> MSRSKRDNNFYSVEIGDSTFTVLKRYQNLKPIGSGAQGIVCAAYDAILERNVAIKKLSRPFQNQTHAKRAYRELVLMKCVNHKNIIGLLNVFTPQKSLEEFQDVYIVMELMDANLCQVIQMELDHERMSYLLYQM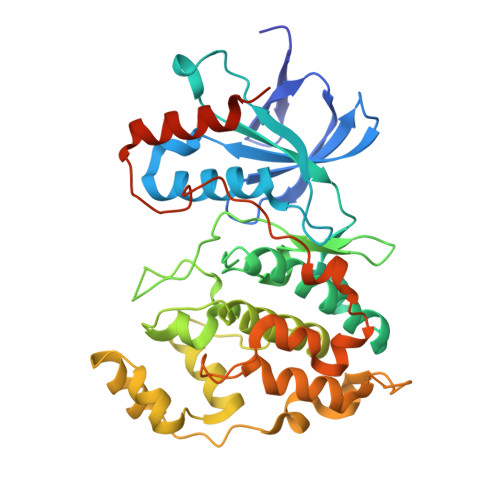LCGIKHLHSAGIIHRDLKPSNIVVKSDCTLKILDFGLARTAGTSFMMTPEVVTRYYRAPEVILGMGYKENVDIWSVGCIMGEMIKGGVLFPGTDHIDQWNKVIEQLGTPCPEFMKKLQPTVRTYVENRPKYAGYSFEKLFPDVLFPADSEHNALKASQARDLLSKMLVIDASKRISVDEALQHPYINVWYDPSEAEAPPPKIPDKQLDEREHTIEEWKELIYKEVMDLPKRPTTLNLFHHHHHH>MATEVTFFDELKIDNKVDIIGNNVRGELPNIWLQYGQFKLKASGGDGTYSWYSENTSIATVDASGKVTLNGKGSVVIKATSGDKQTVSYTIKAP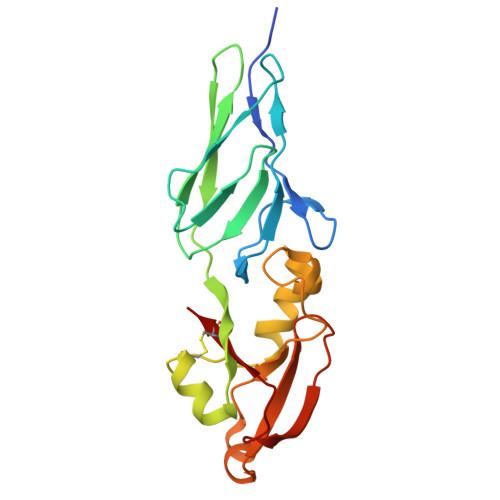SYMIKVDKQAYYADAMSICKNLLPSTQTVLSDIYDSWGAANKYSHYSSMNSITAWIKQTSSEQRSGVSSTYNLITQNPLPGVNVNTPNVYAVCVE[4x]> ATLTAKNLAKAYKGR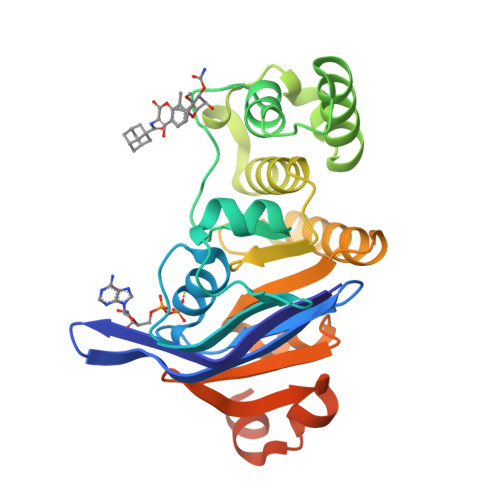RVVEDVSLTVNSGEIVGLLGPNGAGKTTTFYMVVGIVPRDAGNIIIDDDDISLLPLHARARRGIGYLPQEASIFRRLSVYDNLMAVLQIRDDLSAEQREDRANELMEEFHIEHLRDSMGQSLSGGERRRVEIARALAANPKFILLDEPFAGVDPISVIDIKRIIEHLRDSGLGVLITDHNVRETLAVCERAYIVSQGHLIAHGTPTEILQDEHVKRVYLGEDFRLEHHHHHHHH>MKLAVYSTKQYDKKYLQQVNEAFGFELEFFDFLLTEKTAKTANGCEAVCIFVNDDGSRPVLEELKKHGVKYIALRCAGFNNVDLDAAKELGLQVVRVPAYSPEAVAEHAIGMMMTLNRRIHRAYQRTRDANFSLEGLTGFTMHGKTAGVIGTGKIGVAALRILKGFGMRLLAFDPYPSTAALDLGVEYVDLQTLFAESDVISLHCPLTPENYHLLNHAAFDQMKNGVMIINTSRGALIDSQAAIEALKNQKIGSLGMD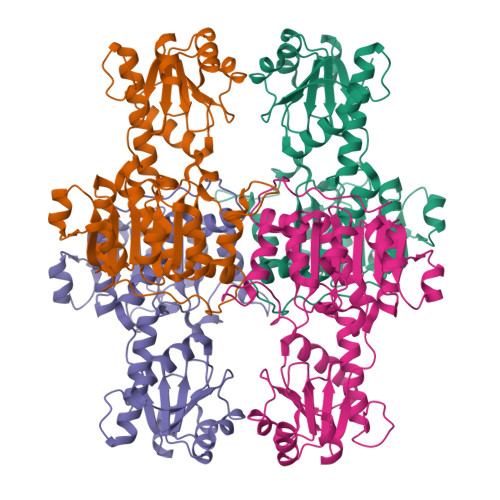VYENERDLFFEDKSVDVIQDDVFRRLSACHNVLFTGHQAFLTAEALISISETTLQNLSQLEKGEACPNALFKSSHHHHHH[4x]>MSLRTQLIAVLIDDYSNPWFIDLIQSLSDVLTPKGYRLSVIDSLTSQAGTDPITSALSMRPDGIIIAQDIPDFTVPDSLPPFVIAGTRITQASTHDSVANDDFRGAEIATKHLIDLGHTHIAHLRVGSGAGLRRFESFEATMRAHGLEPLSNDYLGPAVEHAGYTETLALLKEHPEVTAIFSSNDITAIGALGAARELGLRVPEDLSIIGYD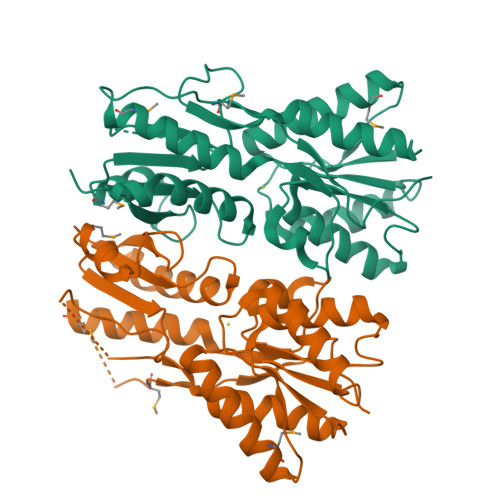NTPLAQTRLINLTTIDDNSIGVGYNAALLLLSMLDPEAPHPEIMHTLQPSLIERGTCAPREGHHHHHH[2x]(2S)-2-(1H-indol-3-yl)hexanoic acid | C14 H17 N O2 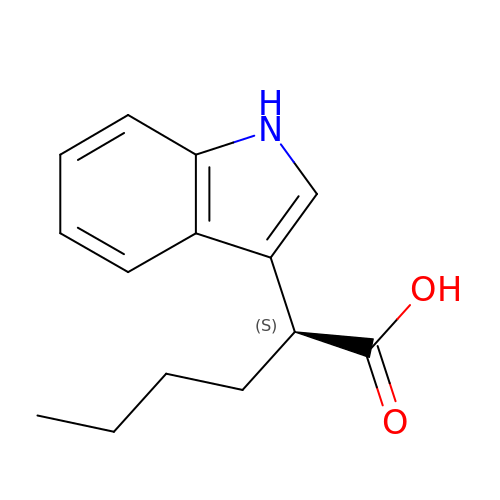| RCBHCHBXRBYJGU-NSHDSACASA-N>MASDASVADSLDTLAAKLIEKAKDLRAGNSTTPQQHEALVGTLKQVQDAVYLPRDDLAAMQMGFVTAAAIRLLLHWKVFEKIPDTGSIRYEELATQVGGDVVIITRICWLLVATGFLVQEGSDR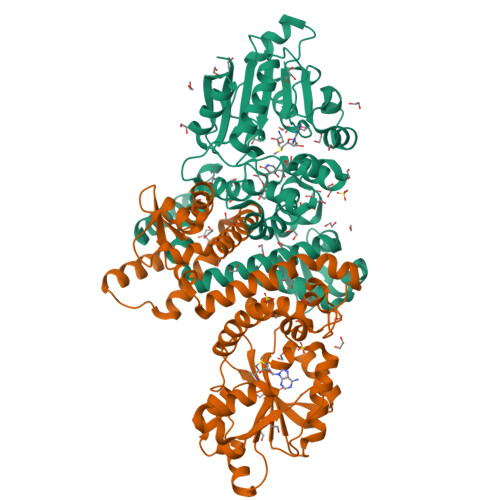VAHTARTRPFAGVNPLRAWWLMGYDEYVPVLLAMPRYYDTYGIKEPTGRLHTIKAFTEGSPELTVGEIMSRHPERTANMLISMSAMASQYPHTGFYDFSWVAPKAAESATRPLIVDIGGAKGWTLQAICKETPEIPISRCVLQDLSGVIQMVQTVGDEDIRSAQLMAIDFHKEQPVQGALVYMIRRILRDFGDDECVSILQHVVAAMAPDSKLLIADTVTGNPPSWFPAMLDFFLSTIGGKERTEEEFRKITARAGLRITGIHYSDKAEFAMIVCEKAEHHHHHH[2x]(2~{S})-2-[2-[[(2~{S})-1,4-bis(oxidanyl)-1,4-bis(oxidanylidene)butan-2-yl]amino]ethylamino]butanedioic 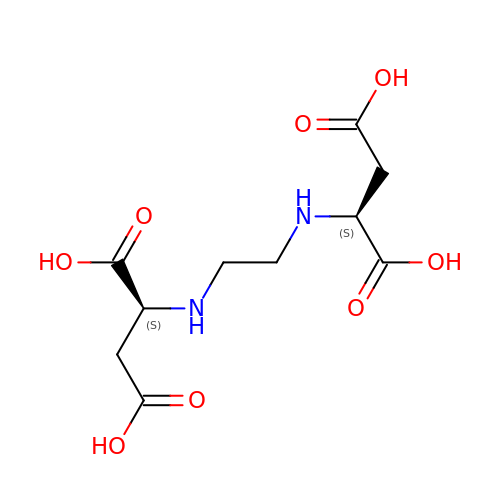acid | C10 H16 N2 O8 | VKZRWSNIWNFCIQ-WDSKDSINSA-N>G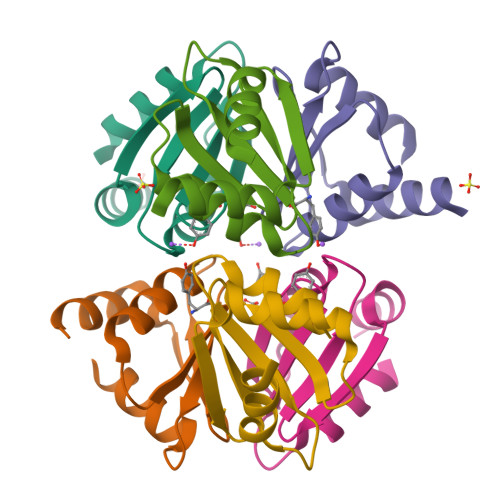TREKLRKMLDDLLVSVDHSGNIAVLRTPPGGAPFLASFIDRVGMEEVVGTIAGDDTVFVLARDPMTGQELGEFLSQRRSGN[2x]>MGDTLTAGQKLERGGSLQSGNGAYTLTLQDDGNLVLYARDKAVWSTGTNGQDVVRAEVQTDGNFVLYTAEKPVWHTDTKGKKEVKLVLQDDRNLVLYAKDGPA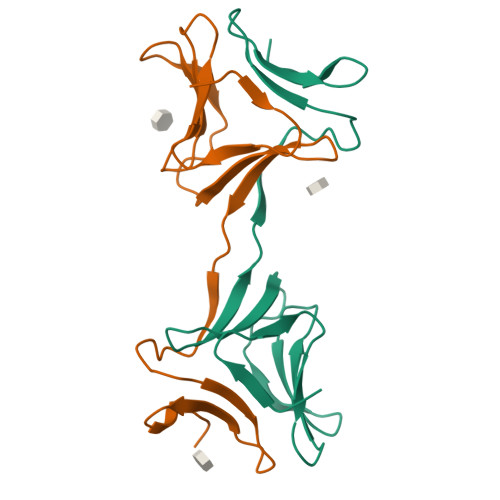WSLEHHHHHH[5x]> MNQTLETGTTTVGITLKDAVIMATERRVTMENFIMHKNGKKLFQIDTYTGMTIAGLVGDAQVLVRYMKAELELYRLQRRVNM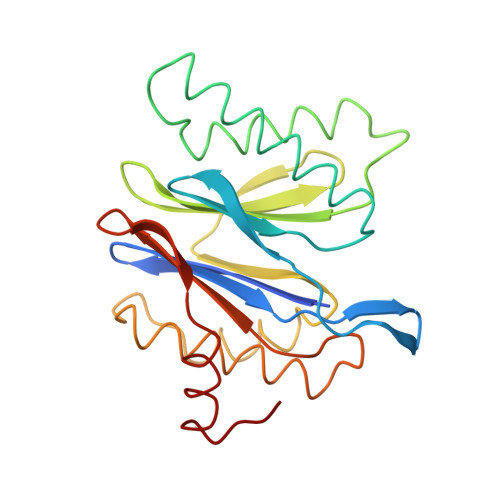PIEAVATLLSNMLNQVKYMPYMVQLLVGGIDTAPHVFSIDAAGGSVEDIYASTGSGSPFVYGVLESQYSEKMTVDEGVDLVIRAISAAKQRDSASGGMIDVAVITRKDGYVQLPTDQIESRIRKLGLIL> MNGVYDVGGTDGLGPINRPADEPVFRAEWEKVAFAMFPATFRAGFMGLDEFRFGIEQMNPAEYLESPYYWHWIRTYIHHGVRTGKIDLEELERRTQYYRENPDAPLPEHEQKPELIEFVNQAVYGGLPRS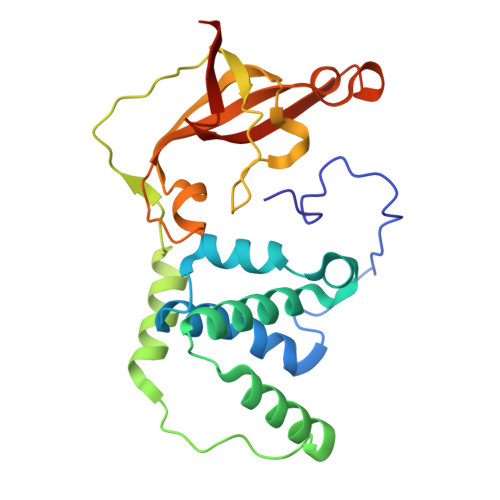REVDRPPKFKEGDVVRFSTASPKGHARRARYVRGKTGTVVKHHGAYIYPDTAGNGLGECPEHLYTVRFTAQELWGPEGDPNSSVYYDCWEPYIELVDTKAAAA>MAQSMYPNEPIVVVGSGCRFPGDANTPSKLWELLQHPRDVQSRIPKERFDVDTFYHPDGKHHGRTNAPYAYVLQDDLGAFDAAFFNIQAGEAESMDPQHRLLLETVYEAVTNAGMRIQDLQGTSTAVYVGVMTHDYETVSTRDLESIPTYSATGVAVSVASNRISYFFDWHGPSMTIDTACSSSLVAVHLAVQQLRTGQSSMAIAAGANLILGPMTFVLESKLSMLSPSGRSRMWDAGADGYARGEAVCSVVLKTLSQALRDGDTIECVIRETGVNQDGRTTGITMPNHSAQEALIKATYAQAGLDITKAEDRCQFFEAHGTGTPAGDPQEAEAIATAFFGHEQVARSDGNERAPLFVGSAKTVVGHTEGTAGLAGLMKASFAVRHGVIPPNLLFDKISPRVAPFYKNLRIPTEATQWPALPPGQPRRASVNSFGFGGTNAHAIIEEYMEPEQNQLRVSNNEDCPPMTGVLSLPLVLSAKSQRSLKIMMEEMLQFLQSHPEIHLHDLTWSLLRKRSVLPFRRAIVGHSHETIRRALEDAIEDGIVSSDFTTEVRGQPSVLGIFTGQGAQWPGMLKNLIEASPYVRNIVRELDDSLQSLPEKYRPSWTLLDQFMLEGEASNVQYATFSQPLCCAVQIVLVRLLEAARIRFTAVVGHSSGEIACAFAAGLISASLAIRIAYLRGVVSAGGARGTPGAMLAAGMSFEEAQEICELDAFEGRICVAASNSPDSVTFSGDANAIDHLKGMLEDESTFARLLKVDTAYHSHHMLPCADPYMQALEECGCAVADAGSPAGSVPWYSSVDAENRQMAARDVTAKYWKDNLVSPVLFSHAVQRAVVTHKALDIGIEVGCHPALKSPCVATIKDVLSGVDLAYTGCLERGKNDLDSFSRALAYLWERFGASSFDADEFMRAVAPDRPCMSVSKLLPAYPWDRSRRYWVESRATRHHLRGPKPHLLLGKLSEYSTPLSFQWLNFVRPRDIEWLDGHALQGQTVFPAAGYIVMAMEAALMIAGTHAKQVKLLEILDMSIDKAVIFDDEDSLVELNLTADVSRNAGEAGSMTISFKIDSCLSKEGNLSLSAKGQLALTIEDVNPRTTSASDQHHLPPPEEEHPHMNRVNINAFYHELGLMGYNYSKDFRRLHNMQRADLRASGTLDFIPLMDEGNGCPLLLHPASLDVAFQTVIGAYSSPGDRRLRCLYVPTHVDRITLVPSLCLATAESGCEKVAFNTINTYDKGDYLSGDIVVFDAEQTTLFQVENITFKPFSPPDASTDHAMFARWSWGPLTPDSLLDNPEYWATAQDKEAIPIIERIVYFYIRSFLSQLTLEERQQAAFHLQKQIEWLEQVLASAKEGRHLWYDPGWENDTEAQIEHLCTANSYHPHVRLVQRVGQHLLPTVRSNGNPFDLLDHDGLLTEFYTNTLSFGPALHYARELVAQIAHRYQSMDILEIGAGTGGATKYVLATPQLGFNSYTYTDISTGFFEQAREQFAPFEDRMVFEPLDIRRSPAEQGFEPHAYDLIIASNVLHATPDLEKTMAHARSLLKPGGQMVILEITHKEHTRLGFIFGLFADWWAGVDDGRCTEPFVSFDRWDAILKRVGFSGVDSRTTDRDANLFPTSVFSTHAIDATVEYLDAPLASSGTVKDSYPPLVVVGGQTPQSQRLLNDIKAIMPPRPLQTYKRLVDLLDAEELPMKSTFVMLTELDEELFAGLTEETFEATKLLLTYASNTVWLTENAWVQHPHQASTIGMLRSIRREHPDLGVHVLDVDAVETFDATFLVEQVLRLEEHTDELASSTTWTQEPEVSWCKGRPWIPRLKRDLARNNRMNSSRRPIYEMIDSSRAPVALQTARDSSSYFLESAETWFVPESVQQMETKTIYVHFSCPHALRVQALGFFYLVQGHVQEGNREVPVVALAERNASIVHVRPDYIYTEADNNLSEGGGSLMVTVLAAAVLAETVISTAKCLGVTDSILVLNPPSICGQMLLHAGEEIGLQVHLATTSGNRSSVSAGDAKSWLTLHARDTDWHLRRVLPRGVQALVDLSADQSCEGLTQRMMKVLMPGCAHYRAADLFTDTVSTELHSGSRHQASLPAAYWEHVVSLARQGLPSVSEGWEVMPCTQFAAHADKTRPDLSTVISWPRESDEATLPTRVRSIDAETLFAADKTYLLVGLTGDLGRSLGRWMVQHGACHIVLTSRNPQVNPKWLAHVEELGGRVTVLSMDVTSQNSVEAGLAKLKDLHLPPVGGIAFGPLVLQDVMLNNMELPMMEMVLNPKVEGVRILHEKFSDPTSSNPLDFFVMFSSIVAVMGNPGQANYSAANCYLQALAQQRVASGLAASTIDIGAVYGVGFVTRAELEEDFNAIRFMFDSVEEHELHTLFAEAVVAGRRAVHQQEQQRKFATVLDMADLELTTGIPPLDPALKDRITFFDDPRIGNLKIPEYRGAKAGEGAAGSKGSVKEQLLQATNLDQVRQIVIDGLSAKLQVTLQIPDGESVHPTIPLIDQGVDSLGAVTVGTWFSKQLYLDLPLLKVLGGASITDLANEAAARLPPSSIPLVAATDGGAESTDNTSENEVSGREDTDLSAAATITEPSSADEDDTEPGDEDVPRSHHPLSLGQEYSWRIQQGAEDPTVFNNTIGMFMKGSIDLKRLYKALRAVLRRHEIFRTGFANVDENGMAQLVFGQTKNKVQTIQVSDRAGAEEGYRQLVQTRYNPAAGDTLRLVDFFWGQDDHLLVVAYHRLVGDGSTTENIFVEAGQLYDGTSLSPHVPQFADLAARQRAMLEDGRMEEDLAYWKKMHYRPSSIPVLPLMRPLVGNSSRSDTPNFQHCGPWQQHEAVARLDPMVAFRIKERSRKHKATPMQFYLAAYQVLLARLTDSTDLTVGLADTNRATVDEMAAMGFFANLLPLRFRDFRPHITFGEHLIATRDLVREALQHARVPYGVLLDQLGLEVPVPTSNQPAPLFQAVFDYKQGQAESGTIGGAKITEVIATRERTPYDVVLEMSDDPTKDPLLTAKLQSSRYEAHHPQAFLESYMSLLSMFSMNPALKLAHVHHHHHH[2x]

The first isolable intermediate of the lovastatin biosynthetic pathway, dihydromonacolin L (DML), is constructed by the highly reducing iterative polyketide synthase (HR-iPKS) LovB, which partners with LovC, an enoyl reductase that acts in trans. In LovB, the β-ketoacyl synthase (KS), malonyl-acetyl transferase (MAT), dehydratase (DH), methyltransferase (CMeT), acyl carrier protein (ACP), and ketoreductase (KR) domains are active, except for the enoyl reductase (ER) domain. LovB terminates with a condensation (CON) domain commonly found in nonribosomal peptide synthetases. In DML biosynthesis by LovB, the initiation and elongation of the intermediate chain are carried out by the KS, MAT, and ACP domains. ß-Ketoacyl modification cycles are also repeated, but the tailoring domain usage during each iteration is highly programmed and permutative.

In this work, we determine the structures of LovB at 2.91 Å and the LovBC complex at 3.60 Å resolution using cryo-electron microscopy. The resolution of the maps enabled us to reliably assign the individual domains, dissect their linker junctions and finally build the atomic models of LovB. The α, β-hydrolase core domain and ferredoxin-like subdomain contained MAT domain have conserved S656, R681, and H763 active site residues, compared with DEBS and mFAS (r.m.s deviation of 1.89 Å and 1.67 Å, respectively). The KS domain adopts an αβαβα structure and contains the conserved C181, H320, and H367 active site residues with r.m.s deviation of 1.57 Å and 1.81 Å, respectively, to DEBS and mFAS. Despite the common fold shared by the KS domains, the substrate tunnels in the KS domains of LovB show differences from those of mFAS and DEBS, highlighted by the disconnection of the PPant pocket from the acyl pocket, possibly due to the hydrophobic interaction of the residue F436 with M132. The NADPH-dependent KR domain adopts the typical Rossmann fold, which belongs to the SDRs (short-chain dehydrogenases/reductases) family. The NADPH binding pocket with bound NADP+ nicotinamide ring can be clearly identified. Each DH monomer of LovB adopts a pseudodimeric hot-dog fold and harbors the conserved active site residues H985, D1174, and Q1178, which are contributed by both hot-dog folds. The S-adenosyl-methionine (SAM)-dependent CMeT domain comprises two subdomains and resembles the homologous modPKS CurJ (r.m.s deviation of 2.39 Å). The ψER adopts the medium-chain dehydrogenases/reductases MDR fold dimer. It lacks the active site residues, and the substrate tunnel is disrupted, leaving no space for substrate and NADP+ cofactor binding.>[2x]MSFDGFFLHHIVEELRSELVNGRIQKINQPFEQELVLQIRSNRQSHRLLLSAHPVFGRIQLTQTTFENPAQPSTFIMVLRKYLQGALIESIEQVENDRIVEITVSNKNEIGDHIQATLIIEIMGKHSNILLVDKSSHKILEVIKHVGFSQNSYRTLLPGSTYIAPPSTESLNPFTIKDEKLFEILQTQELTAKNLQSLFQGLGRDTANELERILVSEKLSAFRNF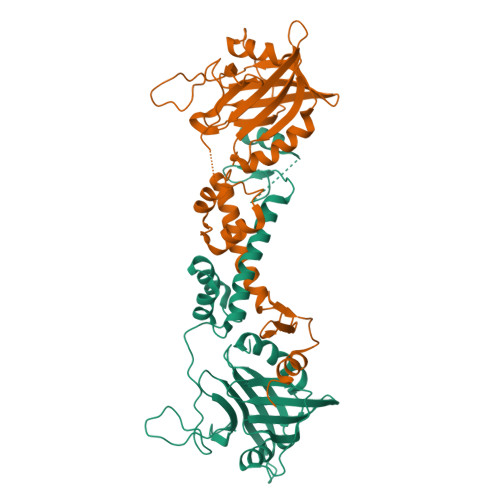FNQETKPCLTETSFSPVPFANQAGEPFANLSDLLDTYYKNKLEHHHHHH docosanoic acid | C22 H44 O2 | 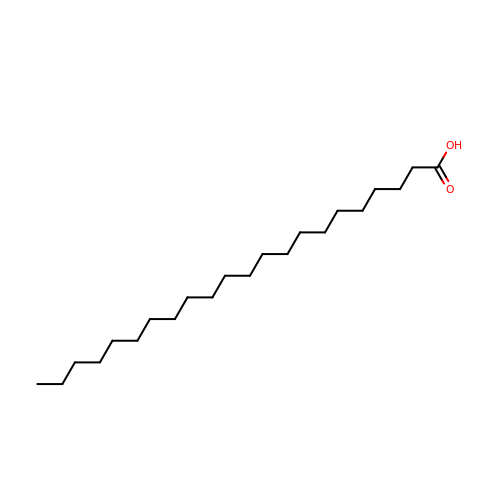UKMSUNONTOPOIO-UHFFFAOYSA-N> L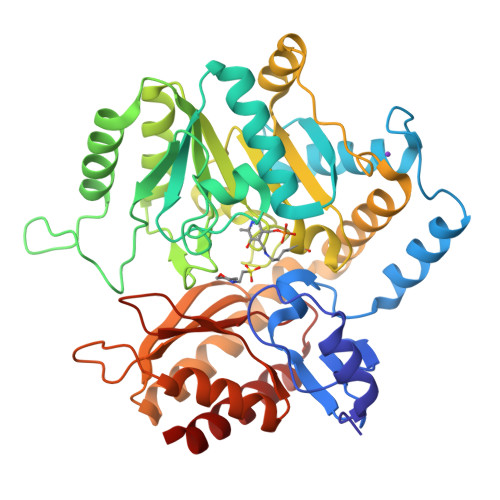NDDATFWRNARHHLVRYGGTFEPMIIERAKGSFVYDADGRAILDFTSGAMSAVLGHCHPEIVSVIGEYAGKLDHLFSEMLSRPVVDLATRLANITPPGLDRALLLSTGAESNEAAIRMAKLVTGKYEIVGFAQSWHGMTGAAASATYSAGRKGVGPAAVGSFAIPAPFTYRPRFERNGAYDYLAELDYAFDLIDRQSSGNLAAFIAEPILSSGGIIELPDGYMAALKRKCEARGMLLILDEAQTGVGRTGTMFACQRDGVTPDILTLSKTLGAGLPLAAIVTSAAIEERAHELGYLFYTTHVSDPLPAAVGLRVLDVVQRDGLVARANVMGDRLRRGLLDLMERFDCIGDVRGRGLLLGVEIVKDRRTKEPADGLGAKITRECMNLGLSMNIVQLPGMGGVFRIAPPLTVSEDEIDLGLSLLGQAIERAL> HMTTPFMSNMTGWTTVNGTWADTIEGKQGRSDGDSFILSSASGSDFTYESDITIKDGNGRGAGALMFRSDKDAKNGYLANVDAKHDLVKFFKFENGAASVIAEYKTPIDVNKKYHLKTEAEGDRFKIYLDDRLVIDAHDSVFSEGQFGLNVWDATAV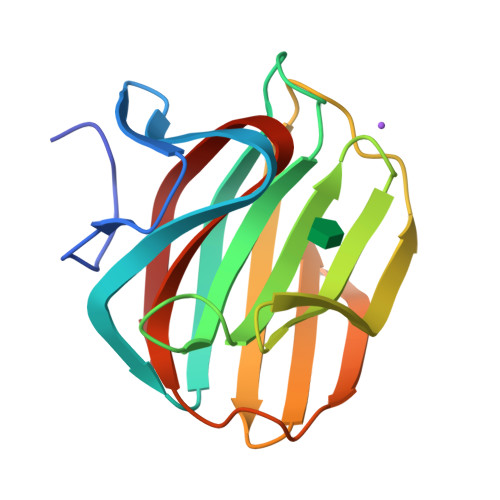FQNVTKES>MGEIYTETLQQTYAWTAGTNIPIKIPRNNFIRKIRVQLIGSISNSGTAAVTLPSAPFPYNLVQTFNLSYEGSKTLYSVSGTGLGILMYYTTKGQNPAYPAPGTSVPASGSVNLNVMWEFDLARFP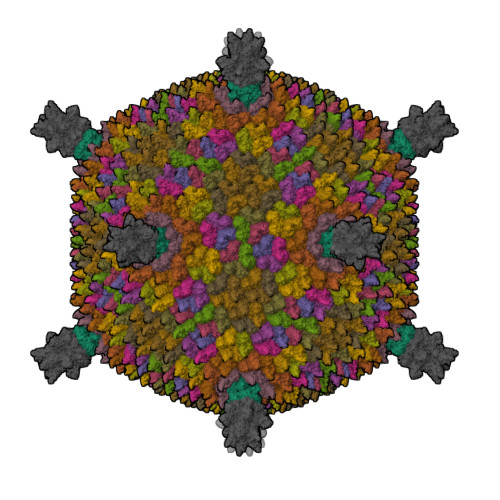ATMVQNIILSILTGQAPSGVSINASFYITITYERVTAQEILSEGGLGADGEMPLATVLPKVIEIPTFNVPASSAPIHVAYLQPGQIYKRQLVYVINSTSGINNTDPTEYELKIVRGVPTDKIKVSWAALQAENQAEYQVAPYSGASAIIDFRKYFNGDLDLTHAPSDSIEYDLALQNQDNVYSLYVSYVLPYYDQLAALPAQVAAIVQQYVARQKRRIKR[15x];> MSVTTLGQSFPANAKVKYYYKLSEKQDLDAFVNSIFVGSYKLKQISYLLYGNTKIVSAPVVPLGPNASIIIDDELQEGLYLIRIKVYNTNSFSVTVTPFFNNNNTMTYSIGANSEFEIYDIFTKEQGNIYYIQLPPGLAILEFSLERVFEKGNRINIPKIIHTSGNGYISFRLRKGTYAIKMPYSYNNTTSTTFTNFQFGTISTSVATIPLVISSIPANGSGSGTFLVYLKITGDYEDVKFSVTYGGGLGVPFTFGLEVEEINELVENTNFVTQSVTLSGSQVTQSILNVQGSGSHLRLKYASVSGLTTAVTQCQLQATNLNRSTTYSTVWDFIAGGSSTPPSWDIREINSIQLVANGGSSTSSVTITLILVYEQIAGELS;> MGEVFKEVKEKFERYKFDVVYVDREYPVSSNNLNVFFEIGERNSFSGLLINEGQAVIDVLLLKKSHEGLSPIPGEGTGIQLSAGQILKFYNVPIAEIIVEYDPSNVSGVSSNVKLKGTIHPLFEVPSQISIENFQPTENYLIYSGFGTSLPQTYTIPANGYLIISITNTSTGNIGQITLTIGSTTMTFNLQTGENKIPVIAGTQITNLTLTSSSAILIYEEVI> MDIKRYCPVTDSELPADHVYFKFRSEIEAAEAYLGLAISEGIKVRETREILDIIDTVYNSLSDPESKLNDFQEKRLNFT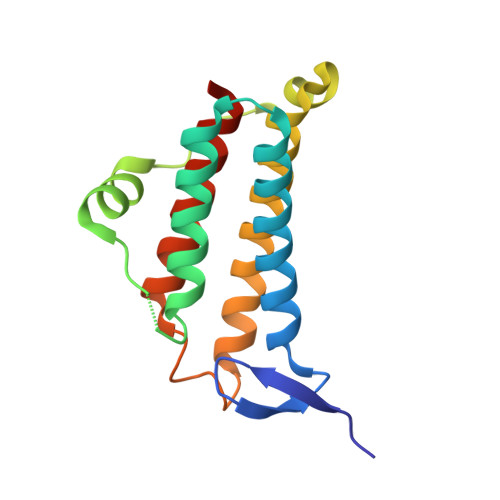EEDWYDIKEKANNGNRWSLYMFLARSAVDSAVYWSYRMKETEEFKEIVKEEMISKLLKAGYVILRESLGEVRL>[4x]MGLSLPKEKGLILCLWSKFCRWFQ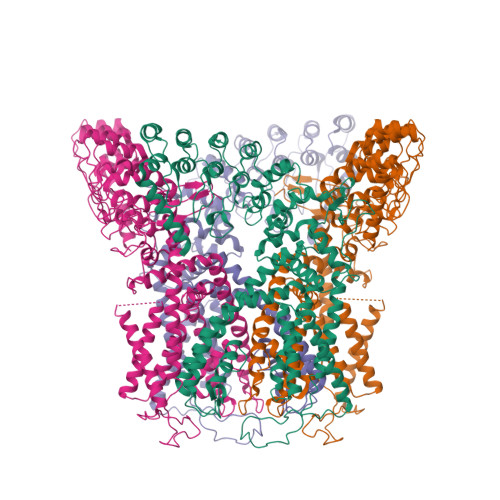RRESWAQSRDEQNLLQQKRIWESPLLLAAKDNDVQALNKLLKYEDCKVHQRGAMGETALHIAALYDNLEAAMVLMEAAPELVFEPMTSELYEGQTALHIAVVNQNMNLVRALLARRASVSARATGTAFRRSPCNLIYFGEHPLSFAACVNSEEIVRLLIEHGADIRAQDSLGNTVLHILILQPNKTFACQMYNLLLSYDRHGDHLQPLDLVPNHQGLTPFKLAGVEGNTVMFQHLMQKRKHTQWTYGPLTSTLYDLTEIDSSGDEQSLLELIITTKKREARQILDQTPVKELVSLKWKRYGRPYFCMLGAIYLLYIICFTMCCIYRPLKPRTNNRTSPRDNTLLQQKLLQEAYMTPKDDIRLVGELVTVIGAIIILLVEVPDIFRMGVTRFFGQTILGGPFHVLIITYAFMVLVTMVMRLISASGEVVPMSFALVLGWCNVMAFARGFQMLGPFTIMIQKMIFGDLMRFCWLMAVVILGFASAFYIIFQTEDPEELGHFYDYPMALFSTFELFLTIIDGPANYNVDLPFMYSITYAAFAIIATLLMLNLLIAMMGDTHWRVAHERDELWRAQIVATTVMLERKLPRCLWPRSGICGREYGLGDRWFLRVEDRQDLNRQRIQRYAQAFHTRGSEDLDKDSVEKLELGCPFSPHLSLPMPSVSRSTSRSSANWERLRQGTLRRDLRGIINRGLEDGESWEYQILVPRGSAAAWSHPQFEK N-(3-{2-[5-chloro-2-(3-chloro-5-cyanophenoxy)phenoxy]ethyl}phenyl)prop-2-enamide 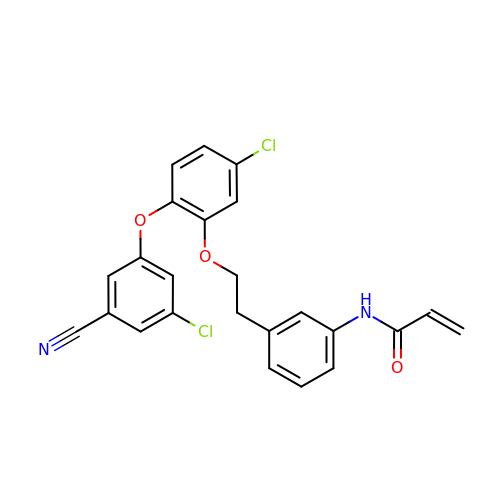| C24 H18 Cl2 N2 O3 | JKEJVDFTNRUUBQ-UHFFFAOYSA-N> TTEENSKSEALLDIPMLEQYLELVGPKLITDGLAVFEKMMPGYVSVLESNLTAQDKKGIVEEGHKIKGAAGSVGLRHLQQLGQQIQSPDLPAWEDNVGEWIEEMKE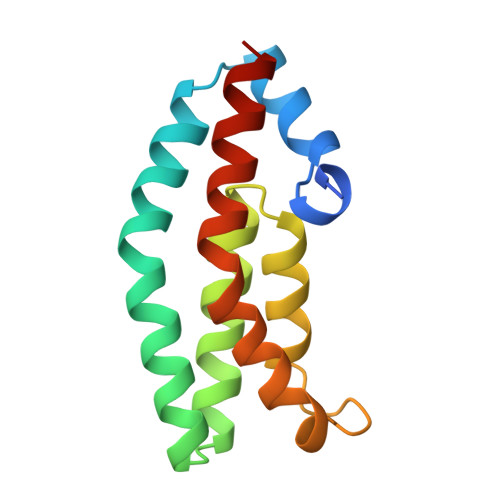EWRHDVEVLKAWVAKATKK> MLRWSRLLREMAPELQLEYIPIIFTRTILGPQGGFAGEERLIKREVAQKYMSEGNAVTPSAEFHQGVWCYNPDSEQYDRFVERNAEFLDFAARKRQWLDVYWRVNTGYLLFGRQSWGQGWLLNCPLRKKDIAQKLWEQYKVRVDPRLIEFREKDRRTGIQDLGHNWCWLYLPGAEELAIDREVYDNKRVKVRMH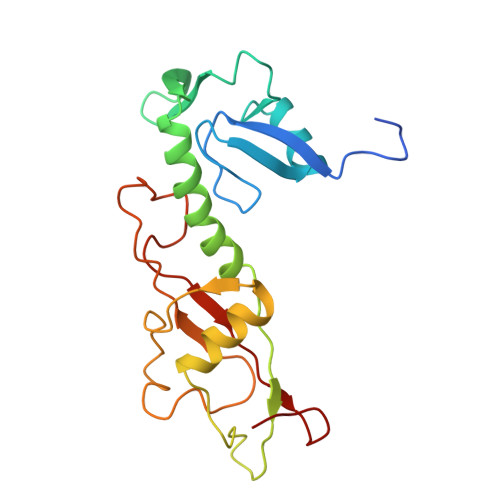IRKMSSYGALY>MEIPVIEPLFTKVTEDIPGAAGPVFDKNGDFYIVAPYVEVNGKPAGEILRIDLKTGKKTVICKPEVNGYGGIPAGCQCDRDANQLFVADMRLGLLVVQTDGTFEEIAKKDSEGRRMQGCAYCAFDYEGNLWITAPAGEVAPADFTISLQEKFGSIYCFTTDGQMIQVDTAFQFPAGIAVRHMNDGRPYQLIVAEQPTKKLWSYDIKGPAKIENKKVWGHIPGTHKGGAAGMDFDEDNNLLVANWGSSHIEVFGPDGGQPKMRIRCPFEKPSALHFKPQTKTIFVTEHENNAVWKFEWQRNGKKQYCETLKFGIF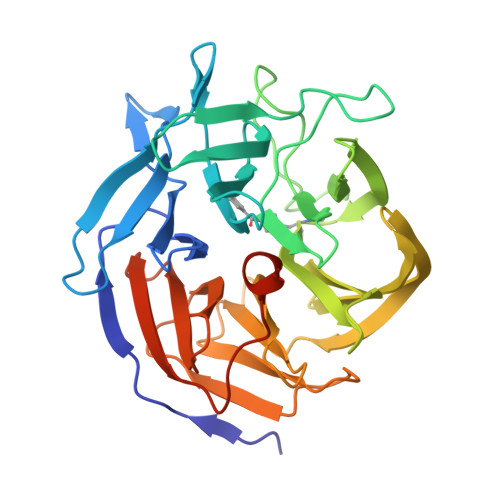GSLEHHHHHH[2x]> ADDEDCCSYEDRREIRHIWDDVWSSSFTDRRVAIVRAVFDDLFKHYPTSKALFERVKIDEPESGEFKSHLVR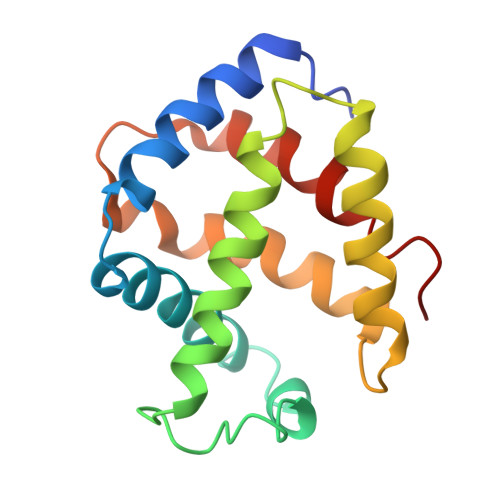VANGLKLLINLLDDTLVLQSHLGHLADQHIQRKGVTKEYFRGIGEAFARVLPQVLSCFNVDAWNRCFHRLVARIAKDLP> GQRWELALGRFWDYLRWVQTLSEQVQEELLSSQVTQELRALMDETMKELKAYKSELEEQLTPVAEETR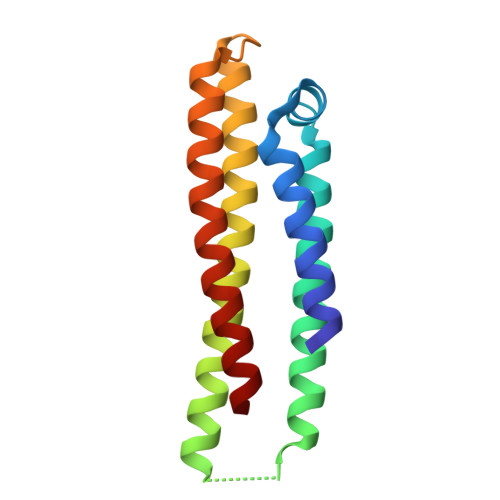ARLSKELQAAQARLGADMEDVRGRLVQYRGEVQAMLGQSTEELRVRLASHLRKLRKRLLRDADDLQKRLAVY>MATTYEEFAAKLDRLDAEFAKKMEEQNKRFFADKPDEATLSPEMKEHYEKFEKMIQEHTDKFNKKMRE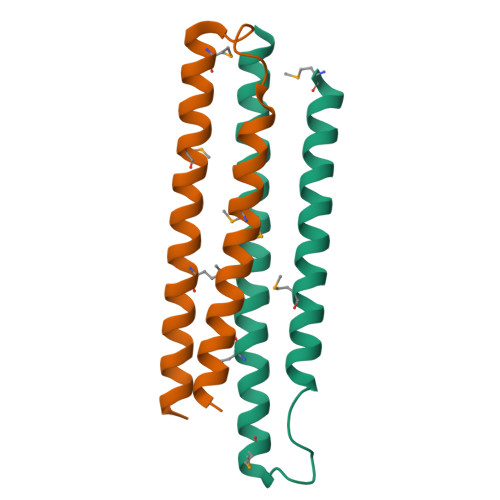HSEHFKAKFAELLEQQKNAQFPGK[2x]> MQRRDFLKY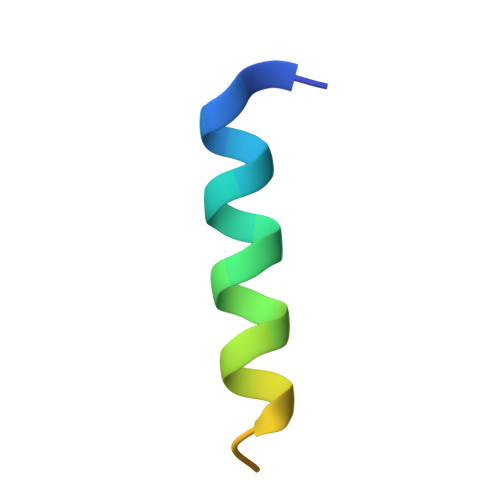SVALGVASALPLWSRAVFA> IAVDGPFGTASEDVFSYEVVMLVGAGIGVTPFA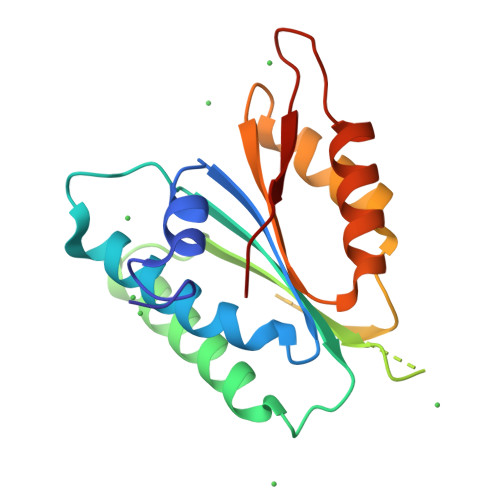SILKSVWYKYCNNATNLKLKKIYFYWLCRDTHAFEWFADLLQLLESQMQERNNAGFLSYNIYLTGWDESQANHFAVHHDEEKDVITGLKQKTLYGRPNWDNEFKTIASQHPNTRIGVFLCGPEALAETLSKQSISNSESGPRGVHFIFNKENF>GAMIVK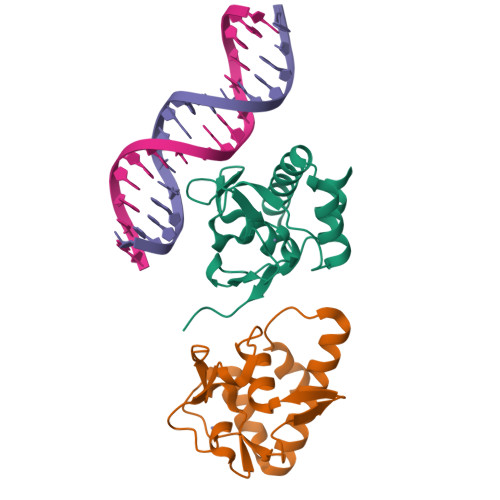RLLGWKKGEQNGQEEKWCEKAVKSLVKKLKKTGQLDELEKAITTQNVNTKCITIPRSLDGRLQVSHRKGLPHVIYCRLWRWPDLHSHHELRAMELCEFAFNMKKDEVCVNPYHYQRVETPVL[2x]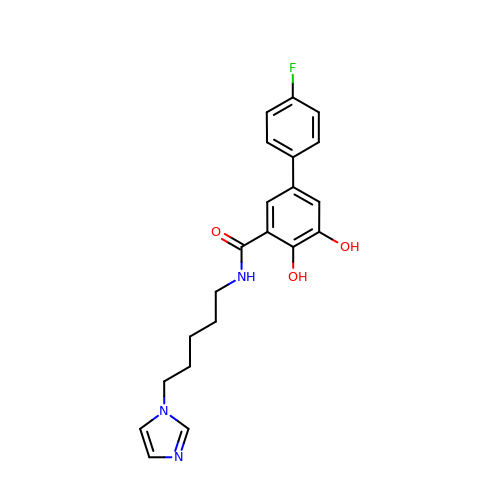5-(4-fluorophenyl)-2,3-dihydroxy-N-(5-imidazol-1-ylpentyl)benzamide | C21 H22 F N3 O3 | WQIGOCFLNCQOJK-UHFFFAOYSA-N>MHHHHHHAKFFATLSQESDASENLIWSGKVDAKNAEGTNTGVALKAGEIITILASGWARNGSENFALTAPQGRIPREGETLTLRNPSLQARLGNENYPVGNHKYRWSVPAEGTLTLFFADGKDQYKDNAGEFSVEVYREADISAAA[4x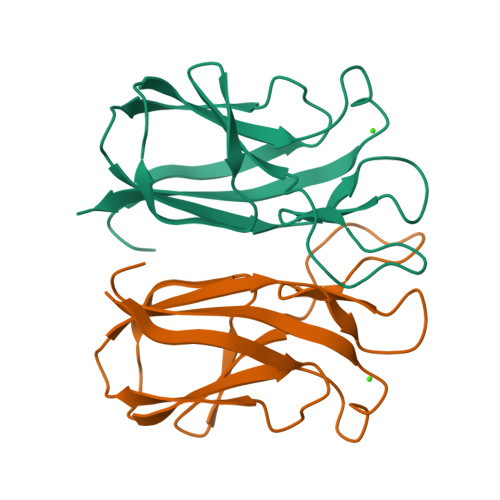]>[4x]MNVVSKTVSLPLKPREFGFFIDGEWRAGKDFFDRSSPAHDVPVTRIPRCTREDLDEAVAAARRAFENGSWAGLAAADRAAVLLKAAGLLRERRDDIAYWEVLENGKPISQAKGEIDHCIACFEMAAGAARMLHGDTFNNLGEGLFGMVLREPIGVVGLITPWNFPFMILCERAPFILASGCTLVVKPAEVTSATTLLLAEILADAGLPKGVFNV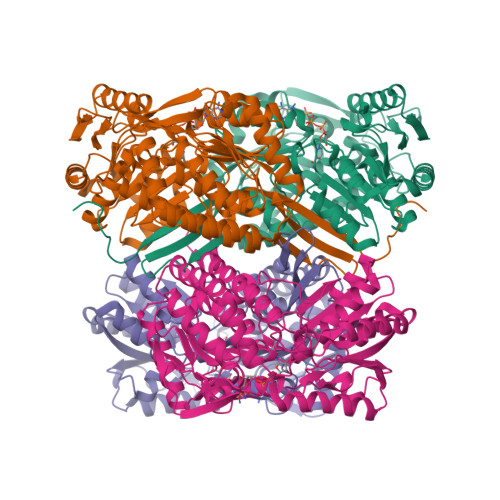VTGTGRTVGQAMTEHQDIDMLSFTGSTGVGKSCIHAAADSNLKKLGLELGGKNPIVVFADSNLEDAADAVAFGISFNTGQCAVSSSRLIVERSVAEKFERLVVAKMEKIRVGDPFDPETQIGAITTEAQNKTILDYIAKGKAEGAKLLCGGGIVDFGKGQYIQPTLFTDVKPSMGIARDEIFGPVLASFHFDTVDEAIAIANDTVYGLAASVWSKDIDKALAVTRRVRAGRFWVNTIMSGGPETPLGGFKQSGWGREAGLYGVEEYTQIKSVHIETGKRSHWISHHHHHH> MCNTYYKRVKFNLFLYTNSIEMELLAVASIIGYGLFSSQQGRETRPDRNRYAEALGSGQGLDEDYDVKPTDMVRKY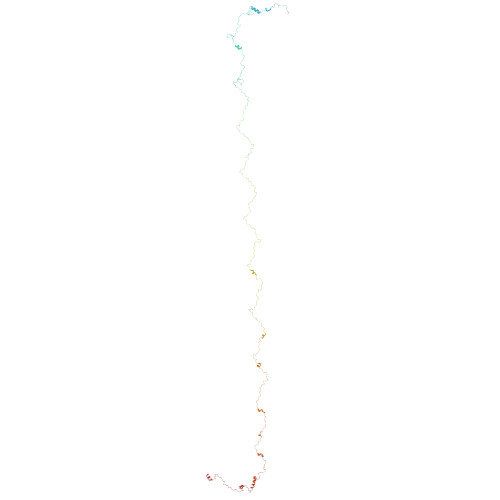RKKAEKRWKKAQVPKESGIITPNMRPSEVMPYFTSGKSMNTNTDYKQRKMELFTGGVLDGHSVSGTYKHKVEAANMFGMTPQGRVTSDGTVGNAPGDTELLKARSVNSHQYNNVLPTEQLRVGPGLGVGPEVAATGGFHQFYRQLPLNINEYKLTQLPGRLVPGGTTTGGKGEIQQIASVNHNPDALVLNYDDRPPEATPNGAILASTQYGKQPRGYAGLRPYEKNYEGIAEADVSALQARYLDQTRGRPRTGDGDTEPIINPNGERDGTGSYVTENMCSMTLESQRGLVNRYITPPGVTGVVQQGGEMRPEFVPETTIREQYEDIYYTGPAGTTVTPTEPMNVVELQPESRHAKRAGQDRAYTPGAGRVNNFAPAAQGAYGLKDHPTYNALQHVVSEPIEQTFLPAAQGDDDRFGTKSNVNNPWGNPASLQIANNQLAANKFNRDVTNTVNLDYDAGQPMKQQNFQPKAWIPNNTDDMKMLPLWKRKQLQAQKNKQQRK>GEKKECWSWESYLEEQKAITAPVSLFQDSQAVTHNKNGFKLGMKLEGIDPQHPSMYFILTVAEVCGYRLRLHFDGYSECH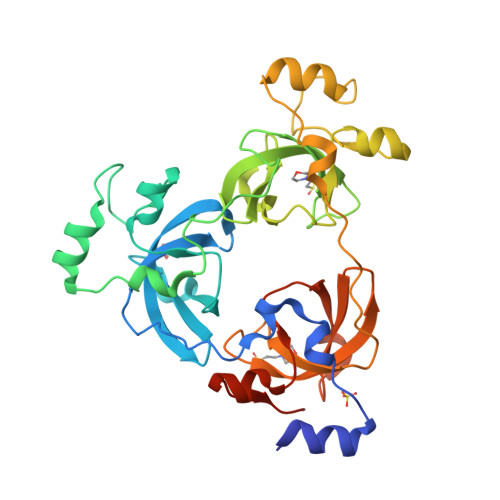DFWVNANSPDIHPAGWFEKTGHKLQPPKGYKEEEFSWSQYLRSTRAQAAPKHLFVSQSHSPPPLGFQVGMKLEAVDRMNPSLVCVASVTDVVDSRFLVHFDNWDDTYDYWCDPSSPYIHPVGWCQKQGKPLTPPQDYPDPDNFCWEKYLEETGASAVPTWAFKVRPPHSFLVNMKLEAVDRRNPALIRVASVEDVEDHRIKIHFDGWSHGYDFWIDADHPDIHPAGWCSKTGHPLQPPLGPREPSSASPGG[3x]>[4x]MERKHHFVLVH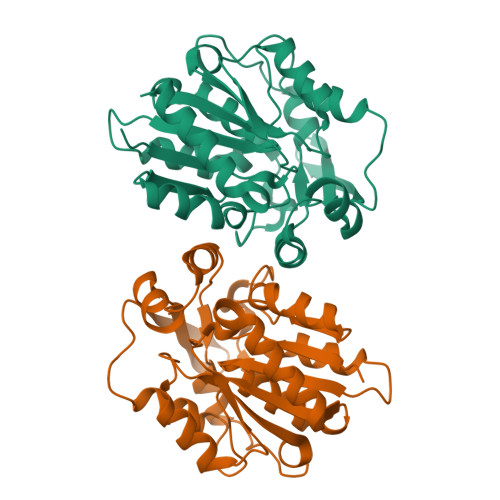NAYHGAWIWYKLKPLLESAGHRVTAVELAASGIDPRPIQAVETVDEYSKPLIETLKSLPENEEVILVGFSFGGINIALAADIFPAKIKVLVFLNAFLPDTTHVPSHVLDKYMEMPGGLGDCEFSSHETRNGTMSLLKMGPKFMKARLYQNCPIEDYELAKMLHRQGSFFTEDLSKKEKFSEEGYGSVQRVYVMSSEDKAIPCDFIRWMIDNFNVSKVYEIDGGDHMVMLSKPQKLFDSLSAIATDYM>[2x]MSVEKIPGYTYGETENRAPFNLEDLKLLKEAVMFTAEDEEYIQKAGEVLEDQVEEILD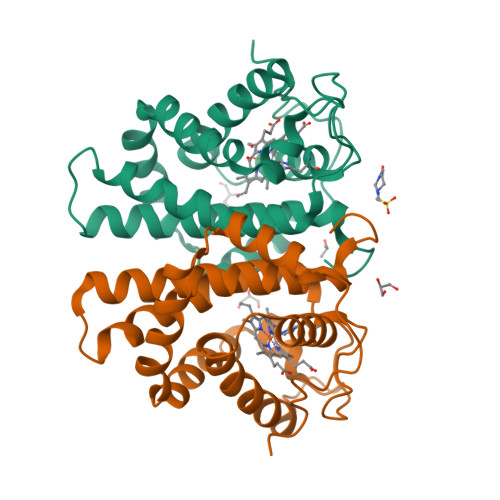TWYGFVGSHPHLLYYFTSPDGTPNEKYLAAVRKRFSRWILDTSNRSYDQAWLDYQYEIGLRHHRTKKNQTDNVESVPNIGYRYLVAFIYPFTATMKPFLARKGHTPEEVEKMYQAWFKATTLQVALWSYPYVKYGDF> GPGSGRVFPHPQDCAQHLMNGDTLSGVYPIFLNGELSQKLQVYCDMTTDGGGWIVFQRRQNGQTDFFRKWADYRVGFGNVEDEFWLGLDNIHRITSQGRYELRVDMRDGQEAAFASYDRFSVEDSRNLYKLRIGSYNGTAGDSLSYHQGRPFSTEDRDNDVAVTNCAMSYKGAWWYKNCHRTNLNGKYGESRHSQGINWYHWKGHEFSIPFVEMKMRPYNHRLMAGRKRQSLQF

PNNs are a condensed form of neural extracellular matrix that include the glycosaminoglycan hyaluronan and extracellular matrix proteins such as aggrecan and tenascin-R (TNR). TNC and TNR share a common domain organization that includes an N-terminal cysteine-rich region responsible for the formation of disulfide-linked multimers, followed by 5-14 epidermal growth factor (EGF)-like domains, 8 to 9 FN repeats, and a C-terminal fibrinogen (Fg)-like domain. Here, we demonstrate that TNR and TNC associate with the single fibronectin type III (FN) domain found in RPTPζ and provide a structural basis of these interactions. Overall, our findings provide novel structural insights in the interactions between RPTPζ and tenascin family members, prove that the formation of a RPTPζ–TNR complex is essential to the assembly of PNNs, and provide a blueprint to explore a potential role for a RPTPζ–TNC complex in neural function.

The Fg region of TNR includes a single Ca2+ ion, and comparison of the bound and free form of human TNR(Fg) indicates that formation of the complex does not induce any significant structural rearrangement. Interestingly, the Fg domain of TNR matches closely with the one found in the lectin tachylectin 5A (RMSD of 1.7 Å over 210 Cα positions) in spite of only 46% sequence identity at the amino acid level. Furthermore, the major contact site in TNR(Fg) overlaps with the N-acetyl-D-glucosamine–binding site found in the Fg domain of tachylectin 5A, and the amide group of Q369 in RPTPζ(FN) occupies a position identical to the acetyl group in the bound carbohydrate. Consistent with this observation, residues in the major contact site of TNR(Fg) are equivalent to those that interact with the N-acetyl-D-glucosamine in the lectin. In fact, this site is also used by the C-terminal Fg domain in fibrinogen to interact with the α chain of fibrin or by the Fg module of angiopoietin-2 to interact with the receptor tyrosine kinase Tie2 (35, 36).> MGKYDGSKLRIGILHARWNAEIILALVLGALKRLQEFGVKRENIIIETVPGSFELPYGSKLFVEKQKRLGKPLDAIIPIGVLIKGSTMHFEYICDSTTHQLMKLNFELGIPVIFGVLTCLTDEQAEARAGLIEGKMHNHGEDWGAAAVEMATKFN;> MEEAELAYLLGELAYKLGEYRIAIRAYRIALKRDPNNAEAWYNLGNAYYKQGRYREAIEYYQKALELDPNNAEAWYNLGNAYYERGEYEEAIEYYRKALRLDPNNADAMQNLLNAKMREELEHHHHHH

We sought to develop a general computational method for de novo designing protein nanoparticles with geometries tailored to present antigens of interest, focusing specifically on the prefusion conformations of the trimeric viral glycoproteins HIV-1 Env (BG505 SOSIP), influenza hemagglutinin (H1 HA), and respiratory syncytial virus (RSV) F (DS-Cav1). In the first step, we de novo designed antigen-tailored trimers, featuring N termini geometrically matched to the C termini of the viral glycoproteins. In the second step, we generated tetrahedral, octahedral, and icosahedral two-component nanoparticles by designing secondary interfaces between a designed trimer (fusion component) and a de novo homo-oligomer (assembly component). This design approach yielded nanoparticles tailored to present 4, 8, or 20 copies of the viral glycoproteins in defined geometries.

Five designs comprising a panel of unique geometric configurations, T33_dn2, T33_dn5, T33_dn10, O43_dn18, and I53_dn5, ran as monodisperse particles of the predicted molecular mass by SEC-MALS and were further investigated by SAXS. The experimental solution scattering curves closely matched the scattering curves computed from the design models for all five designs (metrics in Table 1 and Figure 2—source data 1, bottom five designs). Due to its high valency and production yield, we selected the I53_dn5 nanoparticle to investigate the capacity of its two components to be separately produced and assembled in vitro. The two components of I53_dn5 were re-cloned, expressed, and separately purified (pentameric "I53_dn5A" with His6-tag and trimeric “I53_dn5B”). Nanoparticle assembly appeared to be complete within minutes after equimolar mixing. In order to obtain higher-resolution information, three designs, T33_dn10, O43_dn18, and I53_dn5, representing one nanoparticle from each targeted symmetry (T, O, I), were subjected to cryo-electron microscopy (cryo-EM). The final resolutions of the reconstructed maps for the T33_dn10, O43_dn18, and I53_dn5 nanoparticles were 3.9, 4.5, and 5.3 Å, respectively. Some structural heterogeneity was observed in the cryo-EM data, particularly in the case of I53_dn5. In 2D classification results we generated particle projection averages that range from spherical to ellipsoid shape, indicating some degree of flexibility. Backbone r.m.s.d. values estimated for the asymmetric unit (consisting of a single subunit of component A and component B) were 0.65, 0.98, and 1.3 Å for T33_dn10, O43_dn18, and I53_dn5, respectively.> KSSNEATNITPKHNMKAFLDELKAENIKKFLYNFTQIPHLAGTEQNFQLAKQIQSQWKEFGLDSVELAHYDVLLSYPNKTHPNYISIINEDGNEIFNTSLFEPPPPGYENVSDIVPPFSAFSPQGMPEGDLVYVNYARTEDFFKLERDMKINCSGKIVIARYGKVFRGNKVKNAQLAGAKGVILYSDPADYFAPGVKSYPDGWNLPGGGVQRGNILNLNGAGDPLTPGYPANEYAYRRGIAEAVGLPSIPVHPIGYYDAQKLLEKMGGSAPPDSSWRGSLKVPYNVGPGFTGNFSTQKVKMHIHSTNEVTRIYNVIGTLRGAVEPDRYVILGGHRDSWVFGGIDPQSGAAVVH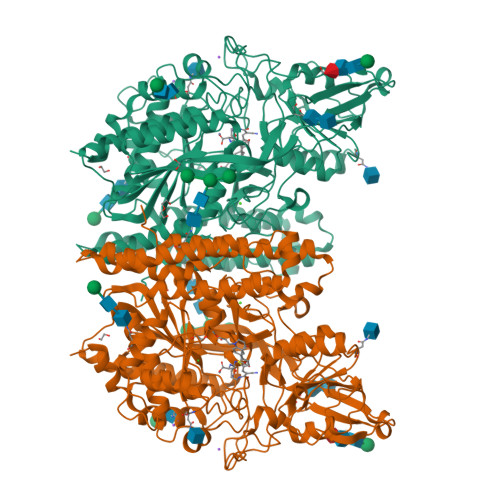EIVRSFGTLKKEGWRPRRTILFASWDAEEFGLLGSTEWAEENSRLLQERGVAYINADSSIEGNYTLRVDCTPLMYSLVHNLTKELKSPDEGFEGKSLYESWTKKSPSPEFSGMPRISKLGSGNDFEVFFQRLGIASGRARYTKNWETNKFSGYPLYHSVYETYELVEKFYDPMFKYHLTVAQVRGGMVFELANSIVLPFDCRDYAVVLRKYADKIYSISMKHPQEMKTYSVSFDSLFSAVKNFTEIASKFSERLQDFDKSNPIVLRMMNDQLMFLERAFIDPLGLPDRPFYRHVIYAPSSHNKYAGESFPGIYDALFDIESKVDPSKAWGEVKRQIYVAAFTVQAAAETLSEVA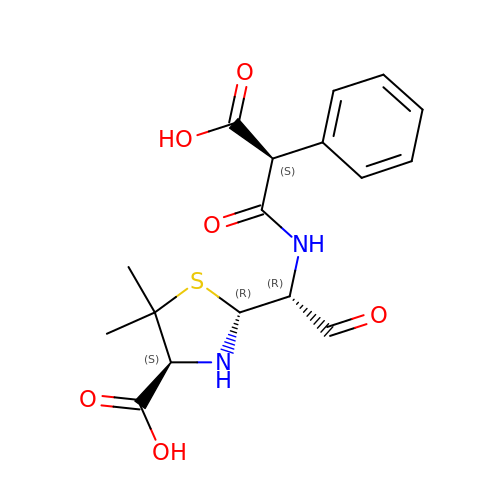(2R,4S)-2-[(1R)-1-{[(2S)-2-carboxy-2-phenylacetyl]amino}-2-oxoethyl]-5,5-dimethyl-1,3-thiazolidine-4-carboxylic acid | C17 H20 N2 O6 S | YABPSSAFCROUQF-OWTLIXCDSA-N>GHMGAFTGKTVLILGGSRGIGAAIVRRFVTDGANVRFTYAGSKDAAKRLAQETGATAVFTDSADRDAVIDVVRKSGALDILVVNAGIGVFGEALELNADDIDRLFKINIHAPYHASVEAARQMPEGGRILIIGSVNGDRMPVAGMAAYAASKSALQGMARGLARDFGPRGITINVVQPGPIDTDANPANGPMRDMLHSLMAIKRHGQPEEVAGMVAWLAG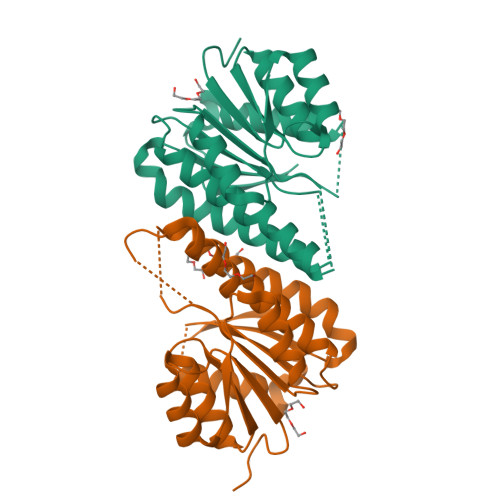PEASFVTGAMHTIDGAFGAG[2x]> MGRDICTLDNVYANNLGMLTKLAHVTVPNLYQDAFF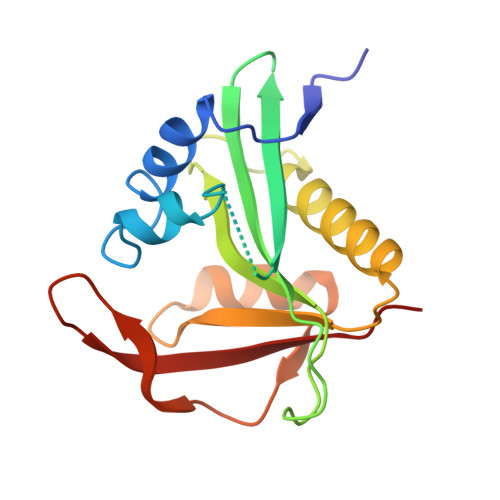SALFAEDSLVAKNKKPSSKKDVHFTQMAYYSEIPVGGLVAKLVPKKQNELSLKGIQIEFLGVLPNYRHKSIGSKLLKFAEDKCSECHQHNVFVYLPAVDDLTKQWFIAHGFEQVGETVNNFIKGVNGDEQDAILLKKHIS> SMSSTSPNLQKAIDLASKAAQEDKAGNYEEALQLYQHAVQYFLHVVKYEAQGDKAKQSIRAKCTEYLDRAEKLKEYLKNKEKKAQKPVKE;> S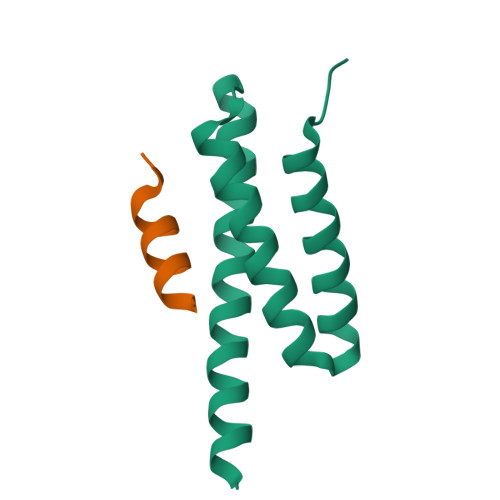TSASEDIDFDDLSRRFEELKKKTW>MEEPEEPADSGQSLVPVYIYSPEYVSMCDSLAKIPKRASMVHSLIEAYALHKQMRIVKPKVASMEEMATFHTDAYLQHLQKVSQEGDDDHPDSIEYGLGYDCPATEGIFDYAAAIGGATITAAQCLIDGMCKVAINWSGGWHHAKKDEASGFCYLNDAVLGILRLRRKFERILYVDLDLHHGDGVEDAFSFTSKVMTVSLHKFSPGFFPGTGDVSDVGLGKGRYYSVNVPIQDGIQDEKYYQICESVLKEVYQAFNPKAVVLQLGADTIAGDPMCSFNMTPVGIGKCLKYILQWQLATLILAGGGYNLANTARCWTYLTGVILGKTLSSEIPDHEFFTAYGPDYVLEITPSCRPDRN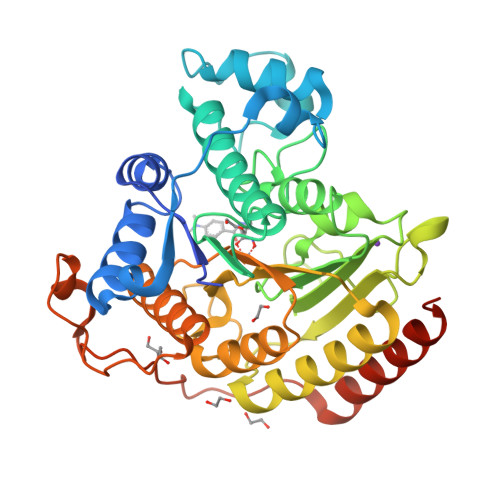EPHRIQQILNYIKGNLKHVVIEGRGSHHHHHH[2x]>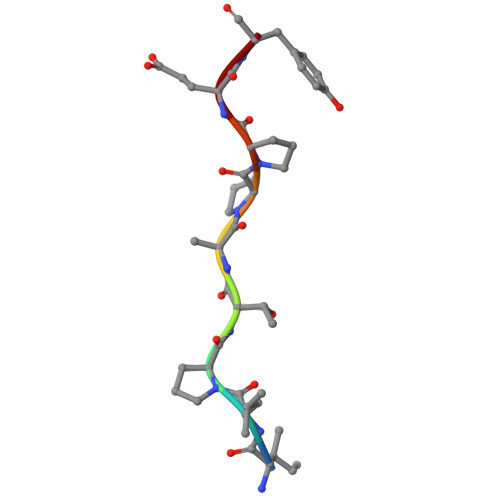 ILPTAPPEY> GAMSSKNEWRKSAIANTLLYLRLKNIYVSADDFVEEQNVYV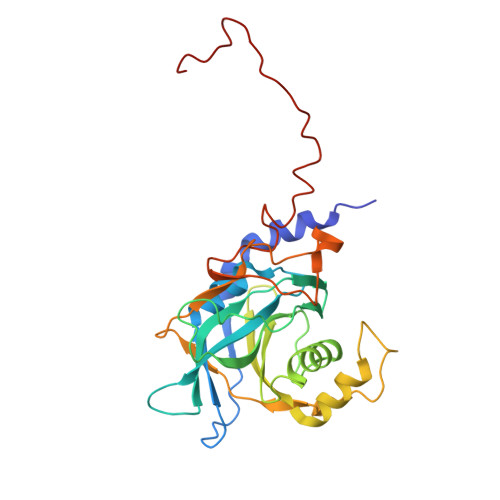LPKNLLKKFIEISDVKIQVAAFIYGMSAKDHPKVKEIKTVVLVPQLGHVGSVQISNIPDIGDLPDTEGLELLGWIHTQTEELKFMAASEVATHSKLFADKKRDCIDISIFSTPGSVSLSAYNLTDEGYQWGEENKDIMNVLSEGFEPTFSTHAQLLLSDRITGNFIIPSGNVWNYTFMGTAFNQEGDYNFKYGIPLEFYNEMHRPVHFLQFSELAGDEELEAEQIDVFS> SNAMKISKVREENRGAKLTVNAKTAVVSENRSQEGILYNDPSRYGKSRKNDEDRDRYIESRLKSSGKLYRIFNEDKNKRETDELQWFLSEIVKKINRRNGLVLSDMLSVDDRAFEKAFEKYAELSYTNRRNKVSGSPAFETCGVDAATAERLKGIISETNFINRIKNNIDNKVSEDIIDRIIAKYLKKSLCRERVKRGLKKLLMNAFDLPYSDPDIDVQRDFIDYVLEDFYHVRAKSQVSRSIKNMNMPVQPEGDGKFAITVSKGGTESGNKRSAEKEAFKKFLSDYASLDERVRDDMLRRMRRLVVLYFYGSDDSKLSDVNEKFDVWEDHAARRVDNREFIKLPLENKLANGKTDKDAERIRKNTVKELYRNQNIGCYRQAVKAVEEDNNGRYFDDKMLNMFFIHRIEYGVEKIYANLKQVTEFKARTGYLSEKIWKDLINYISIKYIAMGKAVYNYAMDELNASDKKEIELGKISEEYLSGISSFDYELIKAEEMLQRETAVYVAFAARHLSSQTVELDSENSDFLLLKPKGTMDKNDKNKLASNNILNFLKDKETLRDTILQYFGGHSLWTDFPFDKYLAGGKDDVDFLTDLKDVIYSMRNDSFHYATENHNNGKWNKELISAMFEHETERMTVVMKDKFYSNNLPMFYKNDDLKKLLIDLYKDNVERASQVPSFNKVFVRKNFPALVRDKDNLGIELDLKADADKGENELKFYNALYYMFKEIYYNAFLNDKNVRERFITKATKVADNYDRNKERNLKDRIKSAGSDEKKKLREQLQNYIAENDFGQRIKNIVQVNPDYTLAQICQLIMTEYNQQNNGCMQKKSAARKDINKDSYQHYKMLLLVNLRKAFLEFIKENYAFVLKPYKHDLCDKADFVPDFAKYVKPYAGLISRVAGSSELQKWYIVSRFLSPAQANHMLGFLHSYKQYVWDIYRRASETGTEINHSIAEDKIAGVDITDVDAVIDLSVKLCGTISSEISDYFKDDEVYAEYISSYLDFEYDGGNYKDSLNRFCNSDAVNDQKVALYYDGEHPKLNRNIILSKLYGERRFLEKITDRVSRSDIVEYYKLKKETSQYQTKGIFDSEDEQKNIKKFQEMKNIVEFRDLMDYSEIADELQGQLINWIYLRERDLMNFQLGYHYACLNNDSNKQATYVTLDYQGKKNRKINGAILYQI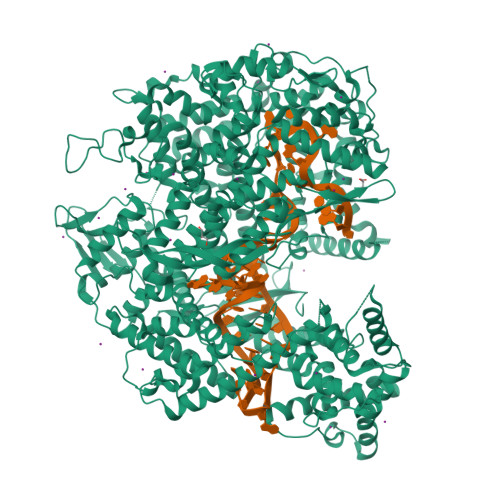CAMYINGLPLYYVDKDSSEWTVSDGKESTGAKIGEFYRYAKSFENTSDCYASGLEIFENISEHDNITELRNYIEHFRYYSSFDRSFLGIYSEVFDRFFTYDLKYRKNVPTILYNILLQHFVNVRFEFVSGKKMIGIDKKDRKIAKEKECARITIREKNGVYSEQFTYKLKNGTVYVDARDKRYLQSIIRLLFYPEKVNMDEMIEVKEKKKPSDNNTGKGYSKRDRQQDRKEYDKYKEKKKKEGNFLSGMGGNINWDEINAQLKN Ricin contains an active A subunit (RTA) and a B subunit (RTB), which promotes retrograde transport into the endoplasmic reticulum (ER). RTA and Stx2A1 are ribosome inactivating proteins (RIPs), which remove a highly conserved adenine base (A4324 in rat) from the sarcin/ricin loop (SRL) of the 28S rRNA, leading to the inhibition of translation, ribotoxic stress, and apoptosis. We showed that RTA is recruited to the SRL by binding first to a conserved sequence at the C-terminal domain (CTD) of ribosomal P-stalk proteins. The X-ray crystal structure analysis showed that RTA binds the last six amino acids of P11 in a hydrophobic pocket at its CTD.

Here we evaluated the second-generation lead compounds that bind at the P-stalk binding site of RTA and identified RU-NT-192, which had 30-fold improved affinity relative to CC10501 and inhibited the cytotoxicity of ricin holotoxin in mammalian cells with no apparent cellular toxicity by itself for the first time. RU-NT-192 had a 32-fold improved Ki value relative to CC10501, while RU-NT-206 showed a 53-fold improved Ki relative to CC10501. The RTA-RU-NT-202, RTA-RU-NT-165, and RTA-RU-NT-192 structures were all determined at 1.8 Å. The RTA-RU-NT-165 and RTA-RU-NT-192 structures were determined in the monoclinic P21 space group with the RTA-RU-NT-202 complex structures solved in the orthorhombic P212121 space group. After superimposing these structures and the structure of RTA with RU-NT-206 (38), the RMSD values range from 0.23 to 0.46 Å, demonstrating no significant conformational changes in the RTA backbone upon binding of these inhibitors. Both RU-NT-165 and RU-NT-192 exhibited more comparable binding patterns, where the carboxylate group within the thiophene ring of each inhibitor formed a salt bridge with the Arg234 side chain and a hydrogen bond with the main chain amide nitrogen of Arg235. Moreover, the ethyl groups at the 2-position within the benzene rings from RU-NT-165 and RU-NT-192 formed distinct hydrophobic interactions with Leu207. In RU-NT-192, the carboxylate is rotated by 26° relative to the thiophene ring, resulting in reduced conjugation and increased electron density on the carboxylate compared to RU-NT-165. This conceivably strengthens the noncovalent interactions between the carboxylate group of RU-NT-192 with Arg234 and Arg235 in RTA. Unlike RU-NT-165, RU-NT-192 formed a π-π stacking interaction between its benzene ring and Phe240 in RTA, further enhancing RU-NT-192's interaction with RTA relative to RU-NT-165 and ultimately supporting its higher inhibitory activity. RU-NT-192 improved the EC50 by 10-fold at 125 μM and by 200-fold at 250 μM and had an EC50 value of 200 pM at 250 μM.

>[2x]SNAMIFPKQYPIINFTTAGATVQSYTNFIRAVRGRLTTGADVRHEIPVLPNRVGLPINQRFILVELSNHAELSVTLALDVTNAYVVGYRAGNSAYFFHPDNQEDAEAITHLFTDVQNRYTFAFGGNYDRLEQLAGNLRENIELGNGPLEEAISALYYYSTGGTQLPTLARSFIICIQMISEAARFQYIEGEMRTRIRYNRRSAPDPSVITLENSWGRLSTAIQESNQGAFASPIQLQRRNGSKFSVYDVSILIPIIALMVYRCAPPPSSQF> GHSFADPASNLG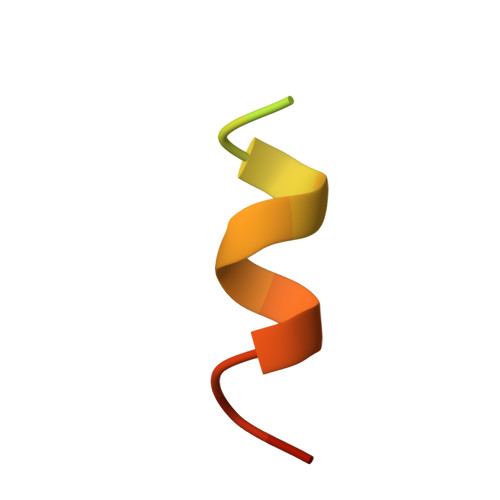LEDIIRKALMGSF> KLV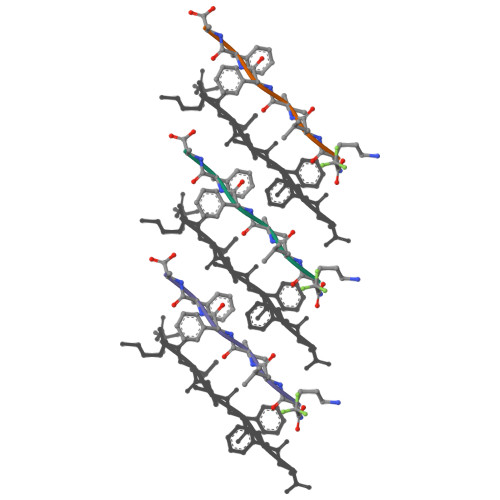FFA> MSLSQIAVRTFHDIRAALLARRELALLDVREEDPFAQAHPLFAANLPLSRLELEIHARVPRRDTPITVYDDGEGLAPVAAQRLHDLGYSDVALLDGGLSGWRNAGGELFRDVNVPSKAFGELVEAERHTPSLAAEEVQALLDARAEAVILDARRFDEYQTMSIPGGISVPGAELVLRVAELAPDPRTRVIVNCAGRTRSIIGTQSLLNAGIPNPVAALRNGTIGWTLAGQQLEHGQTRRFGAISQDTRKAAAQRARAVADRAGVERLDLAGLAQWQDEHDRTTYLLDVRTPEEYEAGHLPGSRSTPGGQLVQETDHVASVRGARLVLVDDDGVRANMSASWLAQMGWQVAVLDGLSEADFSERGAWSAPLPRQPRADTIDPTTLADWLGEPGTRVLDFTASANYAKRHIP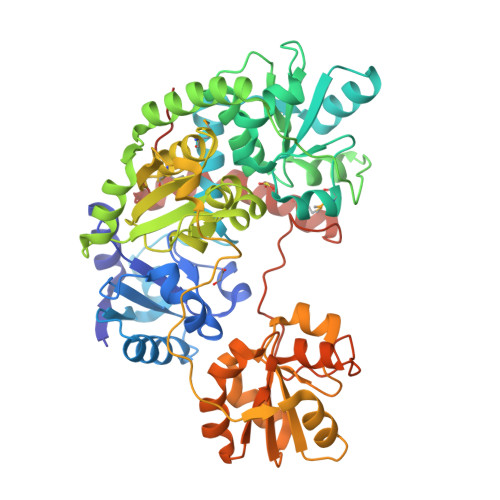GAAWVLRSQLKQALERLGTAERYVLTCGSSLLARFAVAEVQALSGKPVFLLDGGTSAWVAAGLPTEDGESLLASPRIDRYRRPYEGTDNPREAMQGYLDWEFGLVEQLGRDGTHGFFVIEGGSHHHHHH> MIPPLNRYVPALSKNELVKTVTNRDIQFTSFNGKDYPLCFLDEKTPLLFQWFERNPARFGKNDIPIINTEKNPYLNNIIKAATIEKERLIGIFVDGDFFPGQKDAFSKLEYDYENIKVIYRNDIDFSMYDKKLSEIYMENISKQESMPEEKRDCHLLQLLKKELSDIQEGNDSLIKSYLLDKGHGWFDFYRNMAMLKAGQLFLEADKVGCYDLSTNSGCIYLDADMIITEKLGGIYIPDGIAVHVERIDGRASMENGIIAVDRNNHPALLAGLEIMHT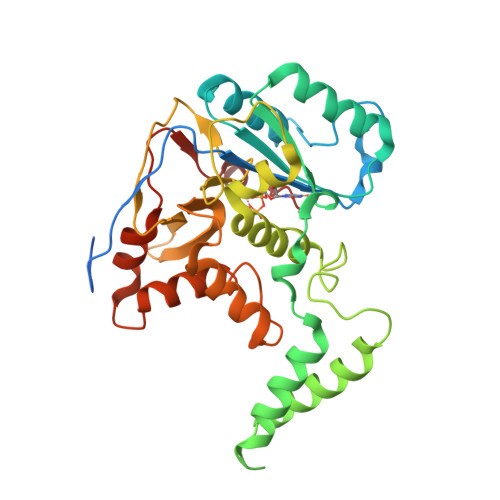KFDADPYSDGVCNGIRKHFNYSLNEDYNSFCDFIEFKHDNIIMNTSQFTQSSWARHVQ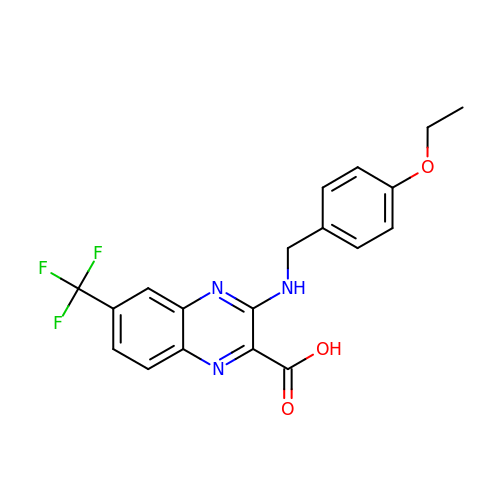3-[(4-ethoxybenzyl)amino]-6-(trifluoromethyl)quinoxaline-2-carboxylic acid | C19 H16 F3 N3 O3 | GGCSQMNZKHRBJW-UHFFFAOYSA-N Finally, L‐sorbosone is further converted into 2‐KLG by a NAD(P)+‐dependent L‐sorbosone dehydrogenase (SNDH). Sequence analysis showed that the SNDH of G. oxydans WSH‐004 belongs to the aldehyde dehydrogenase (ALDH) superfamily (ALDH‐SF). Like other members of ALDH‐SF, SNDH has three typical domains: bridging domain (Red), catalytic domain (Yellow), and cofactor binding domain (Green). The crystal structural analysis found that the SNDH could exist in two different catalytic loop conformations, i.e., the oxidizing SNDH (O‐SNDH) with a closed substrate pocket and the reducing SNDH (R‐SNDH) with an open substrate pocket.

To prove the hypothesis that the catalytic loop is dynamically regulated by a disulfide bond, the catalytic residue Cys296 was mutated into Ala. Mutant C296A was resolved in the form of a homotetramer, which can be described as a dimer of homodimers, and there was no obvious difference in the main chain structure between different subunits. As expected, compared with O‐SNDH, the catalytic loop of the mutant C296A shows a significant difference. Since Cys295 in the catalytic loop cannot form the disulfide bond without Cys296, the catalytic loop enters the enzyme, which makes the substrate pocket present an open conformation. The cofactor pocket is connected with the substrate pocket forming a cofactor‐substrate‐channel, in which the nicotinamide ring of NADP+ is located. In the cofactor pocket of C296A, Thr160, Lys186, and Gln224 stabilize the adenosine ribose. Lys186, Gly219, and the backbone amide groups of Glu189 interact with the 2'‐phosphate group. Trp162 and the backbone amide group of Ser240 hydrogen bonded to the pyrophosphate moiety. Leu263 and Glu294 stabilized the nicotinamide ribose by hydrogen bonding. In the mutant C296A, since Ala296 has no sulfhydryl groups, an enough space can be left for NADP+ to enter the substrate‐cofactor‐channel.

>[4x]MNVVSKTVSLPLKPREFGFFIDGEWRAGKDFFDRSSPAHDVPVTRIPRCTREDLDEAVAAARRAFENGSWAGLAAADRAAVLLKAAGLLRERRDDIAYWEVLENGKPISQAKGEIDHCIACFEMAAGAARMLHGDTFNNLGEGLFGMVLREPIGVVGLITPWNFPFMILCERAPFILASGCTLVVKPAEVTSATTLLLAEILADAGLPKGVFNVVTGTGRTVGQAMTEHQDIDMLSFTGSTGVGKSCIHAAADSNLKKLGLELGGKNPIVVFADSNLEDAADAVAFGISFNTGQCAVSSSRLIVERSVAEKFERLVVAKMEKIRVGDPFDPETQIGAITTEAQNKTILDYIAKGKAEGAKLLCGGGIVDFGKGQYIQPTLFTDVKPSMGIARDEIFGPVLASFHFDTVDEAIAIANDTVYGLAASVWSKDIDKALAVTRRVRAGRFWVNTIMSGGPETPLGGFKQSGWGREAGLYGVEEYTQIKSVHIETGKRSHWISHHHHHH> GSADSKPFVCVNEKDHLPPLDPQADAWYREAAT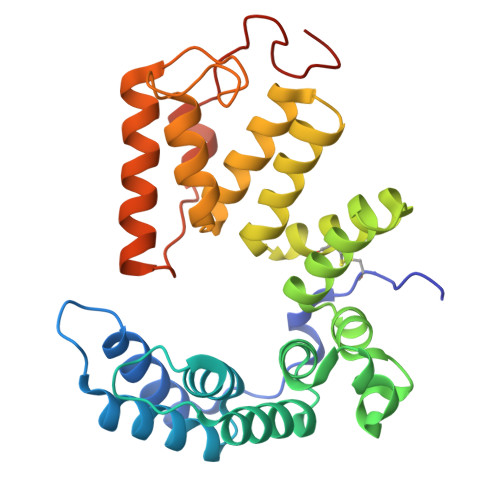LAKPDTLRPWPRIVGLYSKAAERGHWKAMHNLANLYRTGWPGGVEKDTQKALDLYQKMIDLDVPQGFYDMGAMIGNRAGVKNPATDGLTFLDKAASLGNPPALTELGKFYIYVAKKKDLGLAYTHCAASQGYAPASYELGAYYKIVEHNFPKALVYYQVSVSQGGKSAAFFLSRVFGSETPPASAMWYAPDEKLREAYYSIYKKLEADPDLRFPNLIEDYPLPPHPTQGYDADRPDWKPER> MRHFIIDCDTAEDDVLSLYLLLKNNIDVVAVTIVEGNISYEQEVKNALWALEQVNREIPVYPGANKPLLKNYITVEKVHGKGGIGDVTVEPKRLKAQEKHAALAIIDLANEYAGELEFLAISPLTNLALAYLLDNSIVKKIKKVWVMGGAVFGIGNITPVAEFNIWVDPDAAKIVFNAGFDITMIPWDVIINYPVTDEEWNVIKNMKTRMSELYVSMYLHYRQYSSTVQKINGHPHPDAITTAIAIDGSIATRREKRFVVIDNTDNITRGMTLVDRFDADT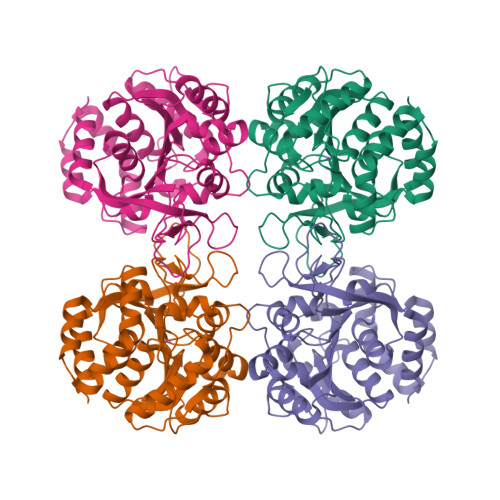SWSDKPNAEIVYEINKKSFMEKIYDLLNWF> DGESTDED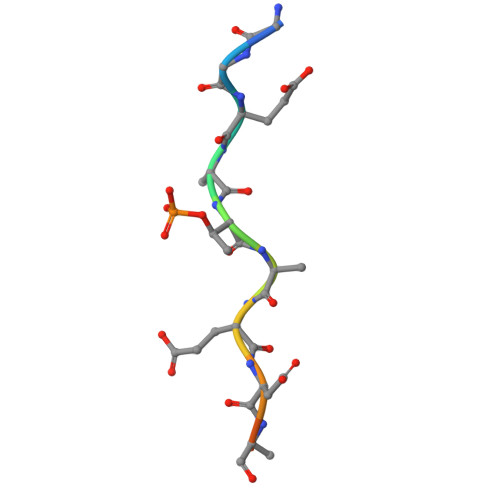DVVS> MAEEEKIIKEEPTNEETEQPEKI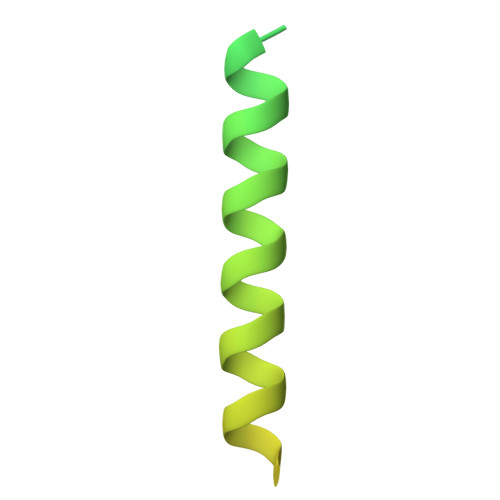ESAEDVVTEPEKEVTEEKSEAFVQLEQRISSLEQRLNNLESQPQPTQESSDPNFEDKTVPTEVDDNQETDGIESSEEIKQMLNL> MENTENSVDSKSIKNLEPKIIHGSESMDSGISLDNSYKMDYPEMGLCIIINNKNFHKSTGMTSRSGTDVDAANLRETFRN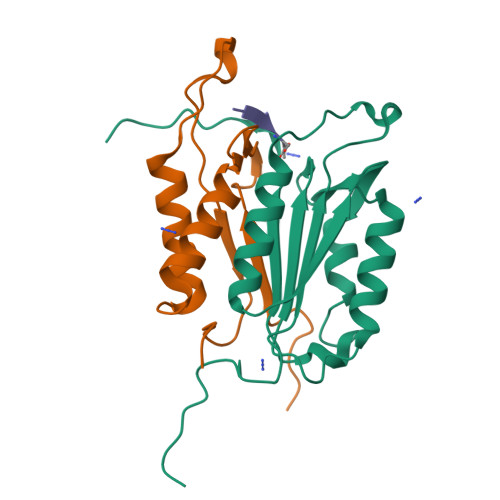LKYEVRNKNDLTREEIVELMRDVSKEDHSKRSSFVCVLLSHGEEGIIFGTNGPVDLKKITNFFRGDRCRELTGKPKLFIIQACRGTELDCGIETD;> SGVDDDMACHKIPVEADFLYAYSTAPGYYSWRNSKDGSWFIQSLCAMLKQYADKLEFMHILTRVNRKVATEFESFSFDATFHAKKQIPCIVSMLTKELYFYH> MTPPKAEKRPYPITTHGDTRVDDYYWLRDDERTDPQVLDYLQAENAFTDAALKPQQALRETLYEEMVARENLYFQSVPYVRHGYRYQTRFEPGNEYAIYVRQPQAESEHWDTLIDGNQRAEQREFYTLGGLEVSPDNQKLAVAEDFLSRRQYDIRFKNLSDDSWTDEVLENTSGSFEWANDSATVYYVRKHAKTLLPYQVYRHVVGTDPQLDELIYEEQDDTFYVGLEKTTSDRFILIHLSSTTTSEILLLDADRADSTPQMFVPRRKDHEYGIDHYHQHFYIRSNKDGKNFGLYQSEQADEAQWQTLIAPRIEVMLEGFSLFRDWLVVEERSEGLTQLRQIHWQSGEVKRIAFDDPTYTTWLAYNPEPETELLRYGYSSMTTPTTLYELNLDSDERVMLKQQEVKNFTPENYRSERVWVKARDGVEVPVSLVYRHDS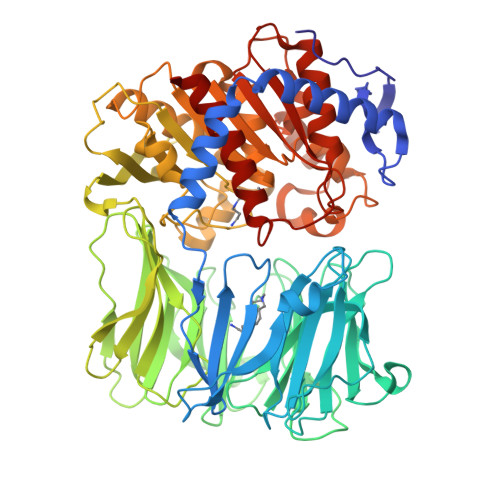FARGTNPLMVYGYGSYGSSMDPAFSASRLSLLDRGFVFVLAHIRGGGELGQLWYEDGKLFKKQNTFNDFIDVTEALIAQGYGDAKRVFAMGGAAGGLLMGAVINQAPELFNGIVAQVPFVDVVTTMLDESIPLTTGEYDEWGNPNQQAYYDYILQYSPYDQVKAQDYPHMLVTTGLHDSQVQYWEPAKWVAKLRELKTDDRQLLLYTDMDSGHGGKSGRFKAYEDIALEYAFILALAE> GSPFNVVPIHNYPELMKDTCALINAEWPRSETARMRSLEASCDSLPCSLVLTTEGM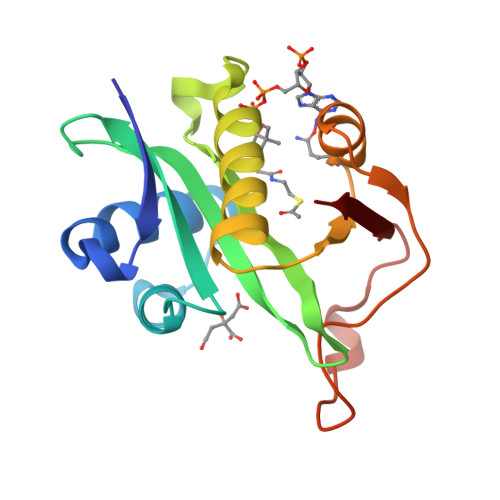CRVIAHLKLSPINSKKKACFVESVVVDKRHRGQGFGKLIMKFAEDYCRVVLDLKTIYLSTIDQDGFYERIGYEYCAPITMYGPRHCELPSLQNAKKKYMKKVL>[4x]NLFQFAKMINGKLGA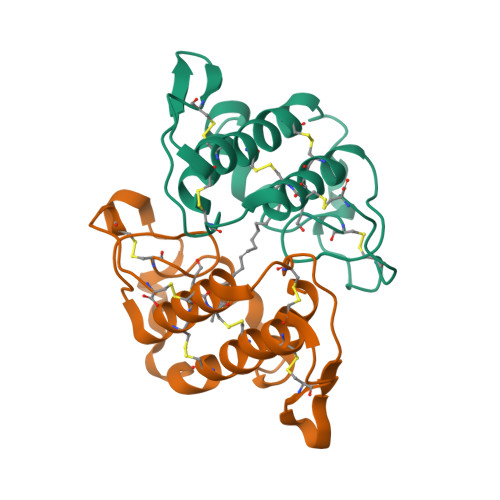FSVWNYISYGCYCGWGGQGTPKDATDRCCFVHDCCYGRVRGCNPKLAIYSYSFKKGNIVCGKNNGCLRDICECDRVAANCFHQNKNTYNKNYKFLSSSRCRQTSEQC> AKEIDVSFVKIEEVIGAGEFGEVYKGRLKLPGKREIYVAIKTLKAGYSEKQRRDFLSEASIMGQFDHPNIIRLEGVVTKSRPVMIITEFMENGALDSFLRQNDGQFTVIQLVGMLRGIAAGMKYLAEMNYVHRDLAARNILVNS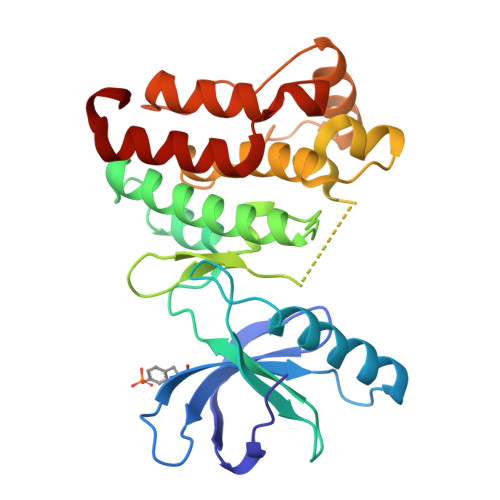NLVCKVSDFGLSRYLQDDTSDPTYTSSLGGKIPVRWTAPEAIAYRKFTSASDVWSYGIVMWEVMSFGERPYWDMSNQDVINAIEQDYRLPPPMDCPAALHQLMLDCWQKDRNSRPRFAEIVNTLDKMIRNPASLK>[2x]TYTTRQIGAKNTLEYKVYIEKDGKPVSAFHDIPLYADKENNIFNMVVEIPRWTNAKLEITKEETLNPIIQDTKKGKLRFVRNCFPHHGYIHNYGAFPQTWEDPNVSHPETKAVGDNDPIDVLEIGETIAYTGQV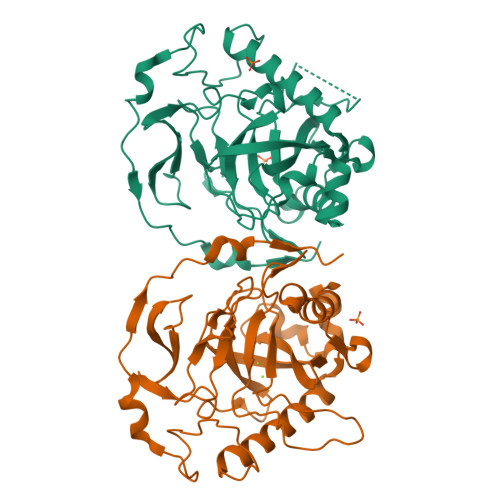KQVKALGIMALLDEGETEWKVIAIDINDPLAPKLNDIEDVEKYFPGLLRATNEWFRIYKIPDGKPENQFAFSGEAKNKKYALDIIKETHDSWKQLIAGKSSDSKGIDLTNVTLPDTPTYSKAASDAIPPASLKADAPIDKSIDKWFFISGSV>[2x]MADSDIVESYARAAGPVHLRVRDIMDPPPGCKVVVNAANEGLLAGSGVCGAIFANATPALAADCRRLAPCPTGEAVATPGHGCG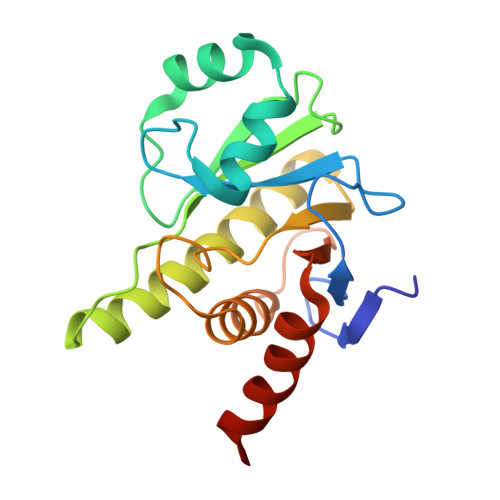YTHIIHAVAPRRPRDPAALEEGEALLERAYRSIVALAAARRWACVACPLLGAGVYGWSAAESLRAALAATRTEPAERVSLHICHPDRATLTHASVLVPLEHHHHHH> MQNSALKAWLDSSYLSGANQSWIEQLYEDFLTDPDSVDANWRSTFQQLPGTGVKPDQFHSQTREYFRRLAKDASRYSSTISDPDTNVKQVKVLQLINAYRFRGHQHANLDPLGLWQQDKVADLDPSFHDLTEADFQETFNVGSFASGKETMKLGELLEALKQTYCGPIGAEYMHITSTEEKRWIQQRIESGRATFNSEEKKRFLSELTAAEGLERYLGAKFPGAKRFSLEGGDALIPMLKEMIRHAGNSGTREVVLGMAHRGRLNVLVNVLGKKPQDLFDEFAGKHKEHLGTGDVKYHMGFSSDFQTDGGLVHLALAFNPSHLEIVSPVVIGSVRARLDRLDEPSSNKVLPITIHGDAAVTGQGVVQETLNMSKARGYEVGGTVRIVINNQVGFTTSNPLDARSTPYCTDIGKMVQAPIFHVNADDPEAVAFVTRLALDFRNTFKRDVFIDLVCYRRHGHNEADEPSATQPLMYQKIKKHPTPRKIYADKLEQEKVATLEDATEMVNLYRDALDAGDCVVAEWRPMNMHSFTWSPYLNHEWDEEYPNKVEMKRLQELAKRISTVPEAVEMQSRVAKIYADRQAMAAGEKLFDWGGAENLAYATLVDEGIPVRLSGEDSGRGTFFHRHAVIHNQSNGSTYT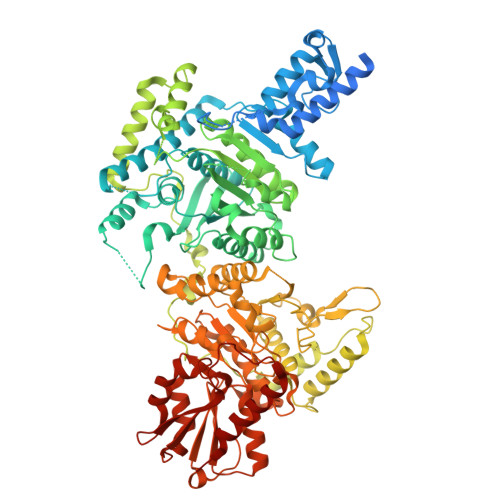PLQHIHNGQGAFRVWDSVLSEEAVLAFEYGYATAEPRTLTIWEAQFGDFANGAQVVIDQFISSGEQKWGRMCGLVMLLPHGYEGQGPEHSSARLERYLQLCAEQNMQVCVPSTPAQVYHMLRRQALRGMRRPLVVMSPKSLLRHPLAVSSLEELANGTFLPAIGEIDELDPKGVKRVVMCSGKVYYDLLEQRRKNNQHDVAIVRIEQLYPFPHKAMQEVLQQFAHVKDFVWCQEEPLNQGAWYCSQHHFREVIPFGASLRYAGRPASASPAVGYMSVHQKQQQDLVNDALNVE>[8x]MSKKFNGKVCLVTGAGGNIGLATALR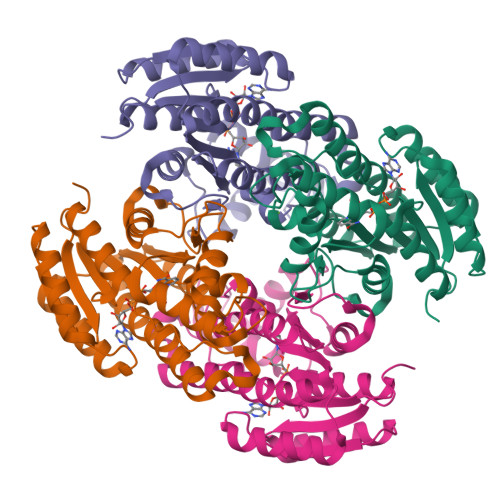LAEEGTAIALLDMNREALEKAEASVREKGVEARSYVCDVTSEEAVIGTVDSVVRDFGKIDFLFNNAGYQGAFAPVQDYPSDDFARVLTINVTGAFHVLKAVSRQMITQNYGRIVNTASMAGVKGPPNMAAYGTSKGAIIALTETAALDLAPYNIRVNAISPGYMGPGFMWERQVELQAKVGSQYFSTDPKVVAQQMIGSVPMRRYGDINEIPGVVAFLLGDDSSFMTGVNLPIAGG>MQWSGARALEALLTVAGELRGPPLQLDTGQLLKIAKRGGVTAVEAVHAWRNALTGAPLNLTPEQVVAIASHDGGKQALETVQRLLPVLCQAHGLTPQQVVAIASHDGGKQALETVQRLLPVLCQAHGLTPEQVVAIASHDGGKQALETVQALLPVLCQAHGLTPEQVVAIASNGGGKQALETVQRLLPVLCQAHGLTPQQVVAIASNGGGKQALETVQRLLPVLCQAHGLTPQQVVAIASRGGKQALETVQRLLPVLCQAHGLTPQQVVAIASNNGGKQALETVQRLLP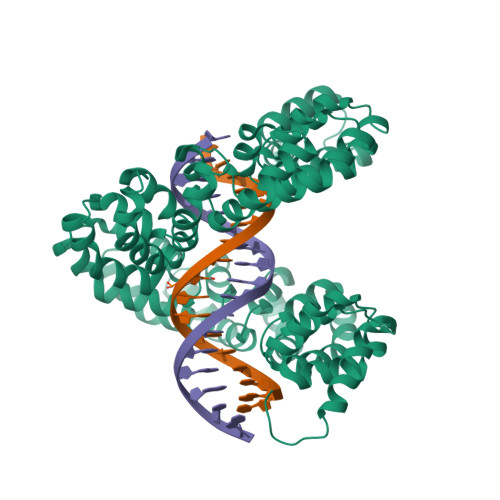VLCQAHGLTPQQVVAIASHDGGKQALETVQRLLPVLCQAHGLTPQQVVAIASNNGGKQALETVQRLLPVLCQAHGLTPEQVVAIASNGGGKQALETVQRLLPVLCQAHGLTPEQVVAIASHDGGKQALETVQRLLPVLCQAHGLTPQQVVAIASNGGGRPALESIVAQLSRPDPALAALTNDHLVALACLGGRPALDAVKKLEHHHHHH[4x]>MLTRNRELTTVLVKNLPKSYNQNKVYKYFKHCGPIIHVDVADSLKKNFRFARIEFARYDGALAAITKTHKVVGQNEIIVSHLTECTLWMTNFPPSYTQRNIRDLLQDINVVALSIRLPSLRFNTSRRFAYIDVTSKEDARYCVEKLNGLKIEGYTLVTKVSNPLEKSKRTDSATLEGREIMIRNLSTELLDENLLRESFEGFGSIEKINIPAGQKEHSFNNCCAFMVFENKDSAERALQMNRSLLGNREISVSLADKKPFLERNEVKRLLASRNSKELETLICLFPLSDKVSP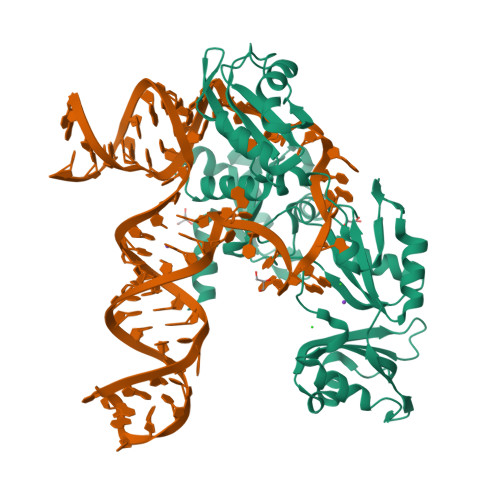SLICQFLQEEIHINEKDIRKILLVSDFNGAIIIFRDSKFAAKMLMILNGSQFQGKVIRSGTINDMKRYYNNQQNHHHHHHH[2x]> MDWEERENLKRLVKTFAFPNFREALDFANRV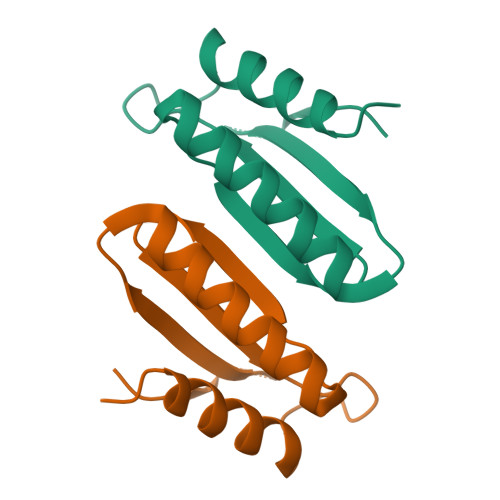GALAERENHHPRLTVEWGRVTVEWWTHSAGGVTEKDREMARLTDALLQR1-(methylsulfonylamino)cyclohexane-1-carboxylic 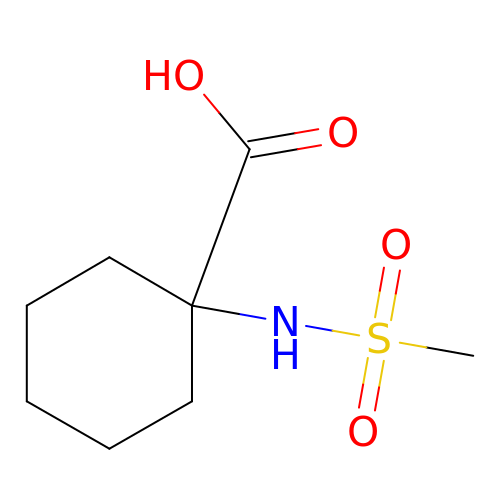acid | C8 H15 N O4 S | RCNDFOGWOOSJJO-UHFFFAOYSA-N> SLLATVGPTGGVKNRLDIVDFVRDEKFFTLYIRALQAIQDKDQSDYSSFFQLSGIHGLPFTPWAKPKDTPTVPYESGYCTHSQVLFPTWHRVYVSIYEQILQEAAKGIAKKFTVHKKEWAQAAEDLRQPYWDTGFALVPPDEIIKLEQVKITNYDGTKITVRNPILRYSFHPIDPSFNGYPNFDTWKTTVRNPDADKKENIPALIGKLDLEADSTREKTYNMLKFNANWEAFSNHGEFDDTHANSLEAVHDDIHGFVGRGAIRGHMTHALFAAFDPIFWLHHSNVDRHLSLWQALYPGVWVTQGPEREGSMGFAPGTELNKDSALEPFYETEDKPWTSVPLTDTALLNYSYPDFDKVKGGTPDLVRDYINDHIDRRYGIKKS;> SLLATVGPTGGVKNRLDIVDFVRDEKFFTLYIRALQAIQDKDQSDYSSFFQLSGIHGLPFTPWAKPKDTPTVPYESGYCTHSQVLFPTWHRVYVSIYEQILQEAAKGIAKKFTVHKKEWAQAAEDLRQPYWDTGFALVPPDEIIKLEQVKITNYDGTKITVRNPILRYSFHPIDPSFNGYPNFDTWKTTVRNPDADKKENIPALIGKLDLEADSTREKTYNMLKFNANWEAFSNHGEFDDTHANSLEAVHDDIHGFVGRGAIRGHMTHALFAAFDPIFWLHHSNVDRHLSLWQALYPGVWVTQGPEREGSMGFAPGTELNKDSALEPFYETEDKPWTSVPLTDTALLNYSYPDFDKVKGGTPDLVRDYINDHIDRRYGIKKSEGGKNPAQDLLSDFKGVTHDHNEDLKMFDWTIQASWKKFELDDSFAIIFYFAADGSTNVTKENYIGSINIFRGTTPTNCANCRTQDNLVQEGFVHLDRFIARDLDTFDPQAVHRYLKEKKLSYKVVADDHSVTLKSLRIRVQGRPLHLPPGVSFPRLDKNIPIVNFDDVLDLVTG

Tyrosinases, bifunctional metalloenzymes, catalyze the oxidation of monophenols and o-diphenols to o-quinones, the precursor compounds of the brown-coloured pigment melanin. Eukaryotic tyrosinases are expressed as inactive zymogens (∼50–80 kDa; latent L-TYR) before being proteolytically activated by the removal of a C-terminal active-site-shielding domain (∼20 kDa). Evidently, the function of the C-terminal domain is not restricted to a shutter function but it may also act as molecular machinery to incorporate copper ions into the active site. Isoform abPPO4 was isolated and extensively purified from the natural source (Agaricus bisporus), which contains a total of six polyphenol oxidases (PPOs).

Here, not only the first crystal structure of the mushroom tyrosinase abPPO4 is presented in its active form (Ser2–Ser383) and in its 21 kDa heavier latent form (Ser2–Thr545), but furthermore the simultaneous presence of both forms within one single-crystal structure is shown. The protein crystallized in space group C2 as a crystallo­graphic heterodimer composed of one polypeptide chain of L-TYR (Ser2–Thr556) and one chain of A-TYR (Ser2–Ser383) as well as two half POM discs ([TeW6O24]6−). The polyoxoanion [TeW6O24]6− with the Anderson–Evans-type structure was deliberately used as a cocrystallization agent to obtain single crystals suitable for X-ray diffraction. The crystal structure of mushroom tyrosinase abPPO4 was solved by combining molecular replacement (MR) and single-wavelength anomalous dispersion (SAD), benefiting from the anomalous scattering signal of the tungsten provided by the cocrystallized POM. The crystal structure of abPPO4 described here with a crystallographic heterodimeric constitution allows a direct comparison between the two active sites of a latent (zymogen) tyrosinase (L-TYR) and its proteolytically activated form (A-TYR). Hence, the CuA site seems to be fixed irrespective of whether or not the C-terminal domain is present. Thus, a coordination of the CuB ion that includes this seventh His282 may be assumed to be an alternative conformation with a minor probability (CuB2; occupancy 0.09). This would result in a somewhat flexible CuB site. The residue Phe454 acts as the substrate placeholder, pointing directly towards CuB at a distance of 4.3 Å (C∊2–CuB). Therefore, an active-site blocking function of the C-terminal domain in a comparable manner can be supported by the data presented here. Thus, each polyoxoanion is bound by a total of eight amino acids from two equivalent monomers (A-TYR abPPO4 or L-TYR abPPO4).> MQELYLLGVVPSRRFEAVVNSLSKTLDGPKTILEFWVVYRPKDVPPNLPRQPDSWLRLCSNIESHDETDTEWSKNTQWSMYLE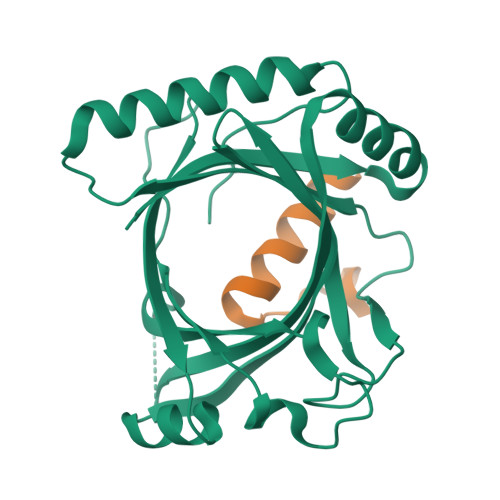GNSEPKREDKCGIRPVNRAKLTNGSVTEFVEKMGYEFSHEYIIQGLEYFFFDTTVRIYQTLIPSQQRSIKPPFHPMNEEQPWILHVYTHVADASNQVAMAKAEANLTKVKTLLSAFCDLKNVRL;> MEEQNANQMLTDILSFMKSGKRAAALEHHHHHH> KRVEGPAPGPETSLWGSQLCSSQ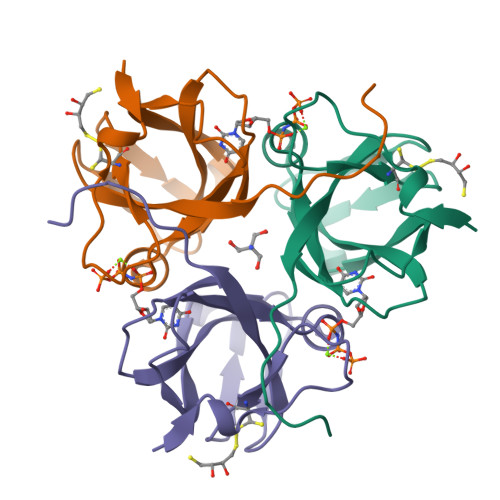QKQPISKLTRATPGSAGLDLCSTSHTVLTPEMGPQALSTGIYGPLPPNTFGLILGRSSITMKGLQVYPGVIDNDYTGEIKIMAKAVNNIVTVSQGNRIAQLILLPLIETDNKVQQPYRGQGSFGSSDIY Kinetoplastid RNA (kRNA) editing takes place in the mitochondria of kinetoplastid protists and creates translatable mRNAs by uridine insertion/deletion. TbRGG2 is a 330 residue protein and contains two main domains, an N-terminal glycine (Gly)-rich region composed of GWG and RG repeats and a C-terminal RNA recognition motif (RRM). Unlike these editing accessory proteins, the T. bruceiRGG2 (TbRGG2) protein is required for editing all nine pan-edited mRNAs. TbRGG2 binds RNA and modulates RNA structure and these functionalities have been shown to be to be essential for its role in kRNA editing.

To address this question we determined crystal structures of the domain, which encompasses residues 203 to 269, from the T. brucei protein. Two apo RRM structures were obtained, one of the RRM(L209M) mutant, which was constructed to aid in crystallographic phasing and one of the WT RRM. Both structures were solved to 1.8 Å to final Rwork/Rfree values of 15.1%/18.7% and 16.5%/19.7%, respectively. The WT RRM structure contains four subunits in the crystallographic asymmetric unit (ASU) and the RRM(L209M) structure contains one. The RRM molecules in the two structures are essentially identical; the Cα atoms of the RRM in both structures can be superimposed with root mean square deviations (rmsds) of 0.4–0.6 Å. The structure shows that the TbRGG2 RRM indeed harbors the characteristic RRM fold composed of a five-stranded anti-parallel β-sheet surrounded by two α-helices (36–37). The TbRGG2 RRM structures revealed no interfaces significant enough to provide stable oligomerization, suggesting the domain itself does not oligomerize. Consistent with this, size exclusion chromatography (SEC) experiments revealed that the RRM domain, even at high concentrations (1 mM), elutes as a monomer.

> GSHMRVQVSGMSDETTWHTLKDHLRQAGEVTFCKVFSGGRAVVEFVTPEDAARAITELQASELEGATLFLR> MHLPNGAQIFVETSRGEEIEATAVTNEKNPVATVASKGDLAKGDYVIVTQSTWAKMVSRVLIVTDAQETSITLAGIDTSDTLVFPAGGTMSFA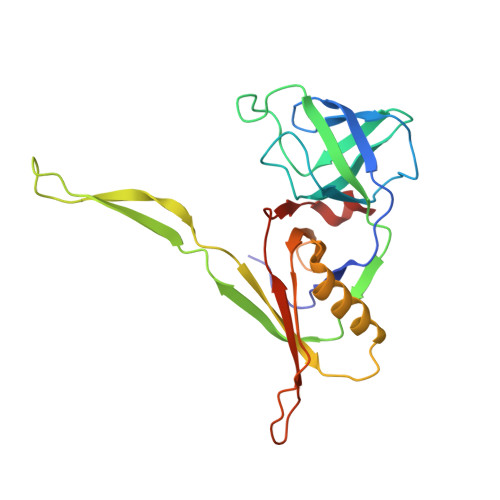KITGWTEIPCVQEIGQDGGEQQYYTYQCLSDDKEQQIPTFKSAISLTYTFAHEFDNPIYQILRKLDSSGQVTAVRMYVPKASEMRMWAGILSFNDIPSTQVNEMETVELAVSLKGDFTFISSTLASPGA>MGSSHHHHHHSSGRENLYFQGHMDAMLLASLVADDRACRIADLGAGAGAAGMAVAARLEKAEVTLYERSQEMAEFARRSLELPDNAAFSARIEVLEADVTLRAKARVEAGLPDEHFHHVIMNPPYNDAGDRRTPDALKAEAHAMTEGLFEDWIRTASAIMVSGGQLSLISRPQSVAEIIAACGSRFGGLEITLIHPRPGED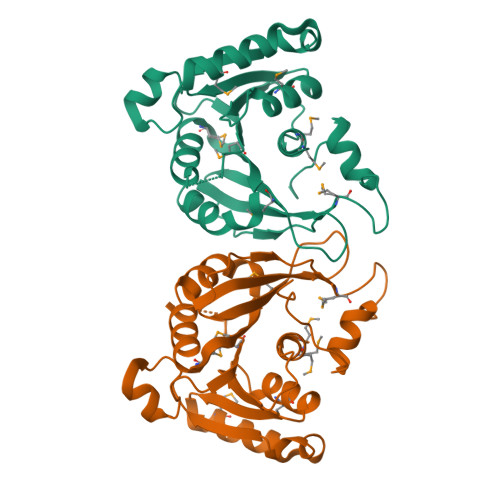AVRMLVTAIKGSRARLTFRAPLIMHETGSHAFTPFVDDLNNGRAAYARNVRAIRTASGS[2x]Here, we reported the enzymatic characterizations and crystal structures of marine bacterial esterases CrmE10 and AlinE4. The results showed that both CrmE10 and AlinE4 belong to the SGNH-hydrolase superfamily and the bacterial lipolytic enzyme GDSL family. The SGNH-hydrolase family, a superfamily that includes the bacterial lipolytic enzyme GDSL family, consists of enzymes possessing four strictly conserved residues, Ser, Gly, Asn, and His, in four conserved blocks, I, II, III, and V, respectively. Among these four residues, Ser and His serve as catalytic residues, and Ser, Gly, and Asn serve as oxyanion hole residues.

AlinE4 had one molecule in an asymmetric unit and was consisted of 11 α-helices (including two 310-helices) and 5 predominant β-strands. AlinE4 had a similar topology with CrmE10, as well as the α9 (Ala168-Ala185) wrapped in other chains and formed a symmetric dimer through the swapped C-terminal domain. For AlinE4, residues Ser13 and Asp162 on chain A and His165 on chain B were in a reasonable position of the catalytic triad, of which hydrogen bonds within the catalytic triad could be formed from Ser13-Oγ to His165-Nε2 and from His165-Nδ1 to Asp162-Oδ1. There was one density map around the catalytic sites in the crystal structure of AlinE4, which turned out to be one Cd2+ evidenced by electrochemistry analysis. In the crystal structure of AlinE4, Cd2+ interacted with residues Ser13 and His165, which were components of the catalytic triad. According to the characterization of AlinE4, Cd2+ had negative impacts on the enzymatic activity of AlinE4, evidenced by only retaining 20% activity at 10 mM CdCl2. The results suggested that Cd2+ might act on activity through (i) blocking proton transfer and (ii) protecting substrates from nucleophile attack. The region of these five sites in CrmE10 formed a negative potential surface; however, the corresponding region was full of positive potential in AlinE4. CrmE10 had about 30% activity at 4 °C and showed no activity above 40 °C, which indicated that CrmE10 was a cold-active enzyme. In contrast, AlinE4 was a mesophilic enzyme with over 32% activity above 60 °C. Interestingly, AlinE4 showed a relatively high thermostability, evidenced by that the enzyme activity was hardly affected after heat treatment at 70 °C for 1 h, and retained 20–40% activity after heat treatment at 100 °C for 1 h. AlinE4 displayed the highest activity (approximately 25.8 U/mg) toward p-NP butyrate (C4) at pH 7.5 and 40 °C (Km, Vmax and kcat of 0.10 mM, 26.9 µmol/mg/min and 25.8 s−1, respectively).

> SMGESRVILAFGDSLFAGYGLDKGESYPAKLETALRSHGINARIINAGVSGDTTAAGLQRIKFVLDSQPDKPELAIVELGGNDLLRGLSPAEARQNLSGILEELQRRKIPILLMGMRAPPNLGAKYQREFDGIYPYLAEKYDAKLVPFFLEAVADRPDLIQKDHVHPTARGVEELVSATSNAVAKALPAKK2-[2-[[2,3-bis(oxidanyl)phenyl]methyl-(2-hydroxy-2-oxoethyl)amino]ethyl-[(2-methylsulfanylphenyl)methyl]amino]ethanoic 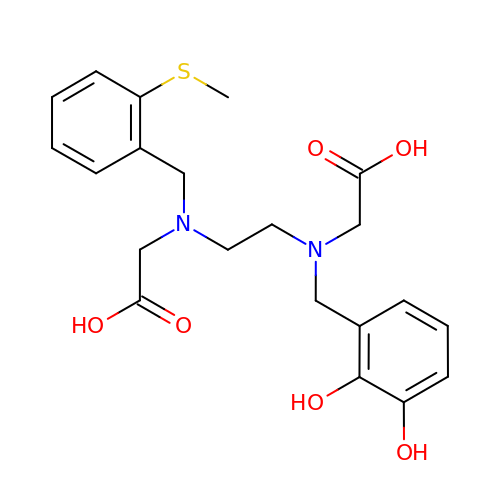acid | C21 H26 N2 O6 S | CCWNBVUPGJNFLR-UHFFFAOYSA-N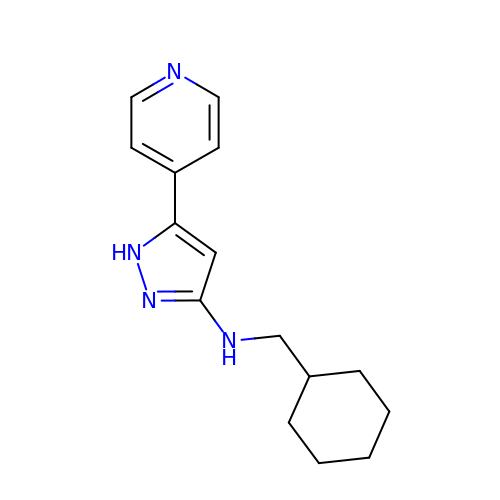N-(CYCLOHEXYLMETHYL)-3-(4-PYRIDYL)-1H-PYRAZOL-5-AMINE | C15 H20 N4 | PAVOZTULRSGNJC-UHFFFAOYSA-N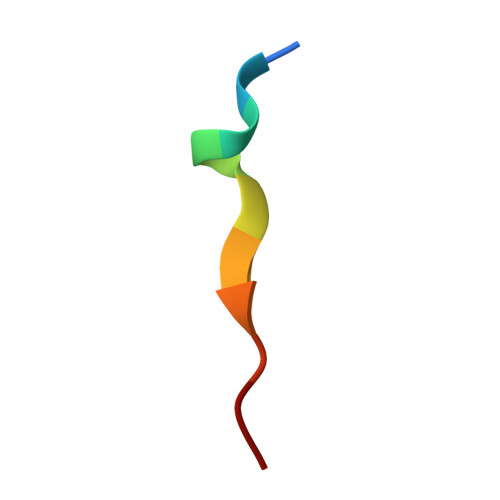> SDLLAWDPLFG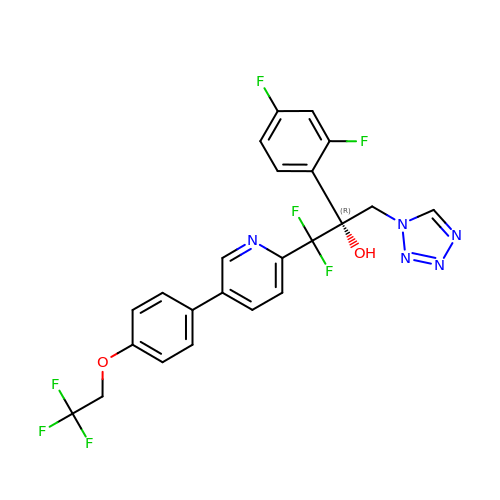(R)-2-(2,4-Difluorophenyl)-1,1-difluoro-3-(1H-tetrazol-1-yl)-1-(5-(4-(2,2,2-trifluoroethoxy)phenyl)pyridin-2-yl)propan-2-ol | C23 H16 F7 N5 O2 | IDUYJRXRDSPPRC-NRFANRHFSA-N>[4x]MRIVQATLEHLDLLAPLFVKYREFYGMLSYPESSRKFLEKRLRRKESVIYLALADEEDRLLGFCQLYPSFSSLSLKRVWILNDIYVAEEARRQLVA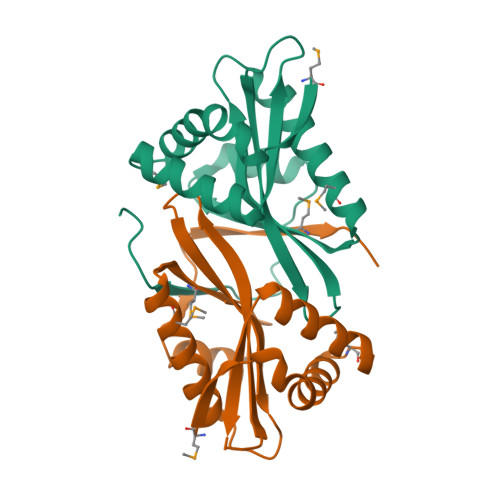DHLLQHAKQMARETHAVRMRVSTSVDNEVAQKVYESIGFREDQEFKNYTLPISDELS3’,5’-cyclic uridine monophosphate (cUMP) and 3’,5’-cyclic cytidine monophosphate (cCMP) have been established as bacterial second messengers in the phage defense system, named pyrimidine cyclase system for anti-phage resistance (Pycsar). Until 2021, scientists reported that a group of bacterial nucleotide cyclases, which utilize UTP, and CTP to synthesize cUMP and cCMP, defend against bacteriophage infection, proving that cUMP, and cCMP are authentic second messengers controlling anti-phage defense in prokaryotes. This anti-phage system, termed pyrimidine cyclase system for antiphage resistance (Pycsar), contains a pyrimidine cyclase PycC and a receptor protein with either transmembrane domain (PycTM) or Toll/interleukin-1 receptor domain (PycTIR). Upon phage infections, produced cyclic mono-pyrimidines activates their receptors PycTM, which disrupts membrane integrity by forming transmembrane-spanning pore, or PycTIR, which deplete NAD+, leading to growth arrests and cell deaths, thus protecting the uninfected bacterial populations, a strategy called “abortive infection”. In this study, we aimed to structurally, and functionally characterize both cUMP- and cCMP-synthesizing PycC and cUMP receptor PycTIR.

The NpPycTIRCNBD crystal structure in the space group P6522 contains only one polypeptide in the asymmetric unit (from residues 1–91 and 98–140), forming a central six-stranded antiparallel β-barrel surrounded by five α-helices. The loop connecting β5 and β6 and the last ten amino acids at the C-terminus are unresolved in the NpPycTIRCNBD crystal structure owing to structural flexibility. Structural comparison of NpPycTIRCNBD with PsPycTIRCNBD shows r.m.s.d. of 1.1 and 0.9 for 116 and 117 Cα pairs, respectively. ITC results showed that both NpPycTIRCNBD and PsPycTIRCNBD bind tightly to cUMP with nanomolar affinity at a 1:1 binding stoichiometry. cUMP also showed strong binding to AhPycTIRCNBD and SmPycTIRCNBD with dissociation constant (KD) of 8.2 × 10−7 M and 2.7 × 10−7 M, demonstrating that PycTIR is a high-affinity cUMP receptor. The Pycsar system has two types of downstream effectors: PycTM and PycTIR. This study provides the structural information regarding the bacterial PycTIR in both apo and cUMP-bound states. The binding of cUMP by PycTIR is probably an example of induce-fit: cUMP induces the conformational change of the helix and promotes the dimerization of PycTIRCNBD, which subsequently strengthens the recognition of cUMP by inter-subunit contact, including the specificity-determining residue N143.

> MGALLDRFSGDEKKGRLIEAVCGQDLVANDKDLAEQIVAAGVLQEIADGDVIIKQGDWDDDLFLILAGKMQITINGRPQTVREAGTHVGELTGTSPARPRTATVSAIGEALVLRLKRTVLDEITRDSPAYLKRMLDVVAGRLDERNKGIGQTNDIPRIFVISSSEKIGVANEIVRNLDSKEIAVQLWDKGTFGISDYPISSLMDAIESSDFTIAVVGADDTLTMRGETHQVARDNVHLEFGISLGVLGRRRSMLLVCADDGVRLPSDAAGLTTLRYRTGSDDEMKRTVRNACIEAKEHIEKEGVFTDRRAR>[16x]MASWSHPQFEKGAETAVPNSSSMEFIVYLAGEIHSNWREEIKEKTKSLKLPIT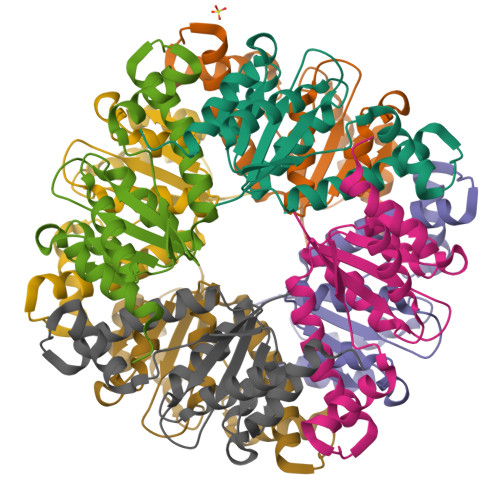FVGPMENHDRSDNIGEEIMGVQPNAVLKDDKASDINNFRTAVLMNKADFVIALFGEKYKQWNTAMDASYAIAKGKPLIIIRPESLHHPLKELSNKANITVETVNQAIKALSYLFETE> MRGSHHHHHHGMASHITYDLPVAIEDILEAKKRLAGKIYKTGMPRSNYFSERCKGEIFLKFENMQRTGSFKIRGAFNKLSSLTEAEKRKGVVACSAGNHAQGVSLSCAMLGIDGKVVMPKGAPKSKVAATC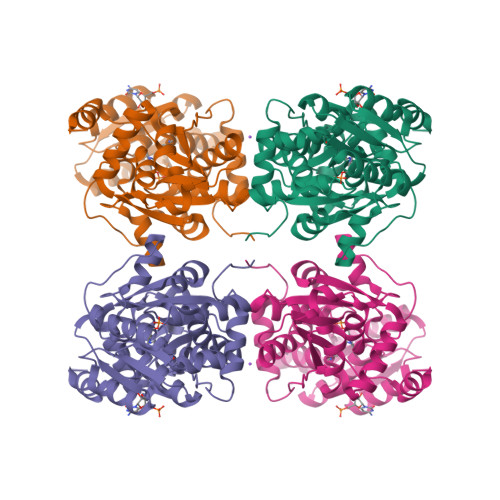DYSAEVVLHGDNFNDTIAKVSEIVETEGRIFIPPYDDPKVIAGQGTIGLEIMEDLYDVDNVIVPIGGGGLIAGIAIAIKSINPTIKVIGVQAENVHGMAASYYTGEITTHRTTGTLADGCDVSRPGNLTYEIVRELVDDIVLVSEDEIRNSMIALIQRNKVITEGAGALACAALLSGKLDSHIQNRKTVSIISGGNIDLSRVSQITGLVDA>MRGSHHHHHHGSMDKDCEMKRTTLDSPLGKLELSGCEQGLHEIKLLGKGTSAADAVEVPAPAAVLGGPEPLMQCTAWLNAYFHQPEAIEEFPVPALHHPVFQQESFTRQVLWKLLKVVKFGEVISYQQLAALAGNPKAARAVGGAMRGNPVPILI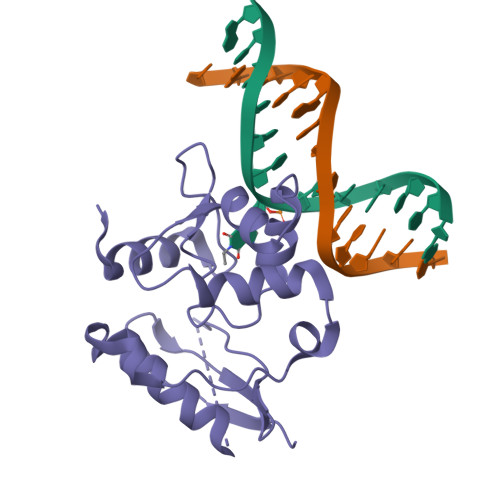PCHRVVCSSGAVGNYSGGLAVKEWLLAHEGHRL[2x]>MTVFVDHKIEYMSLEDDAELLKTMAHPMRLKIVNELYKHKALNVTQIIQILKLPQSTVSQHLCKMRGKVLKRNRQGLEIYYSINNPKVEGIIKLLNPIQ[4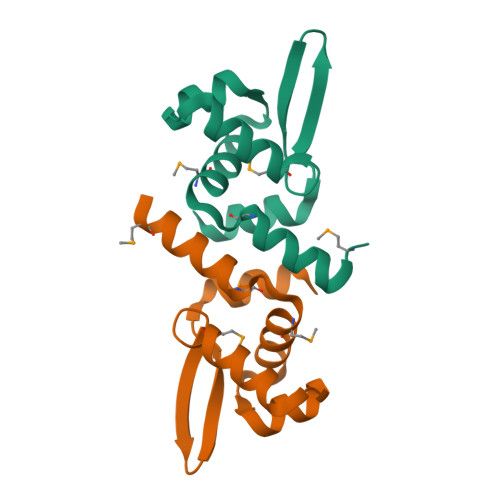x]4-[(E)-C-methyl-N-oxidanyl-carbonimidoyl]benzene-1,3-diol | C8 H9 N O3 | 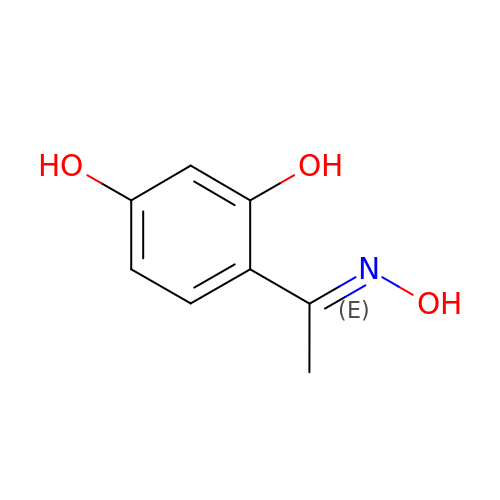FQPRUMXSHZSJGM-WEVVVXLNSA-N>SELDAKLNKLGVDRIAISPYKQWTRGYMEPGNIGNGYVTGLKVDAGVRDKSDNNVLDGIVSYDRAETKNAYIGQINMTTAS[3x];>[3x]XFTGVQGRVIGYDILRSPEVDKAKPLFTETQWDGSELPIYD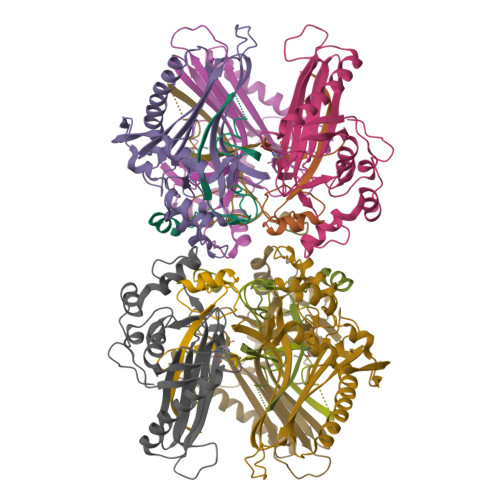AKPLQDALVEYFGTEQDRRHYPAPGSFIVCANKGVTAERPKNDADMKPGQGYGVWSAIAISFAKDPTKDSSMFVEDAGVWETPNEDELLEYLEGRRKAMAKSIAECGQDAHASFESSWIGFAYTMMEPGQIGNAITVAPYVSLPIDSIPGGSILTPDKDMEIMENLTMPEWLEKMGYKSLSANNALKY>GPGSMMSLPVEAVKEFLLKLQDDICHAIEAEDEQATFMEDKWTREGGGGGRTR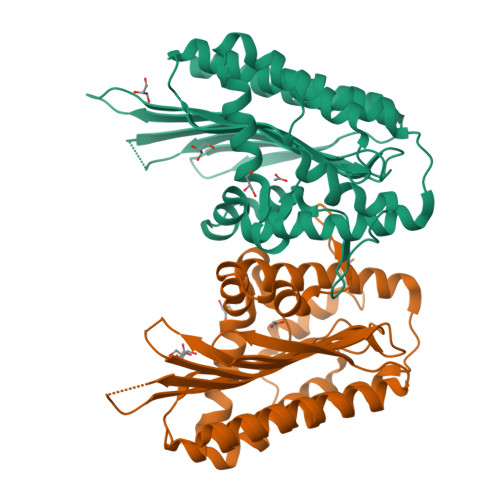VIANGAVIEKGGVNFSHVYGKGLPGSSTERHPDMAGCNYQAMGVSLVIHPKNPHVPTSHANVRLFVAEKEGKEPVWWFGGGFDLTPYYAVEEDCYYFHHVAQELCRPFGADVYERFKAWCDEYFFIPHRNEARGIGGLFFDDLNEWPFEKCFAFMQAVGKGFIDAYIPIVNRRKNTPYTEQQVEFQEFRRGRYAEFNLVIDRGTKFGLQSGGRTESILMSLPPRARWGYNWHPEPGTPEARLTEYFLTKKQWV[2x]> MQCVLAKIVADKAIWVEA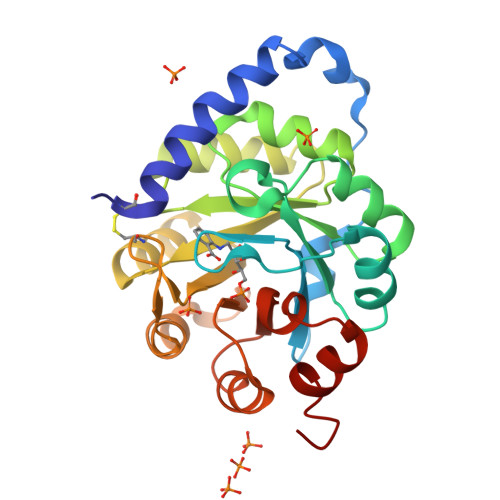RKQQQPLASFQNEVQPSTRHFYDALQGARTAFILECKKASPSKGVIRDDFDPARIAAIYKHYASAISVLTDEKYFQGSFNFLPIVSQIAPQPILCKDFIIDPYQIYLARYYQADACLLMLSVLDDDQYRQLAAVAHSLEMGVLTEVSNEEEQERAIALGAKVVGINNRDLCDLSIDLNRTRELAPKLGHNVTVISESGINTYAQVRELSHFANGFLIGSALMAHDDLHAAVRRVLLGENKV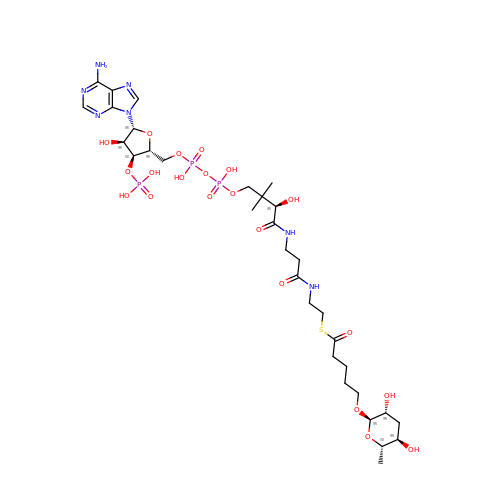~{S}-[2-[3-[[(2~{R})-4-[[[(2~{R},3~{S},4~{R},5~{R})-5-(6-aminopurin-9-yl)-4-oxidanyl-3-phosphonooxy-oxolan-2-yl]methoxy-oxidanyl-phosphoryl]oxy-oxidanyl-phosphoryl]oxy-3,3-dimethyl-2-oxidanyl-butanoyl]amino]propanoylamino]ethyl] 5-[(2~{R},3~{R},5~{R},6~{S})-6-methyl-3,5-bis(oxidanyl)oxan-2-yl]oxypentanethioate | C32 H54 N7 O21 P3 S | OJJVYBQJWBBERR-XKGQWQQESA-N> MKSSHHHHHHENLYFQSSSDFVGTHGQLQVIGNQLCNQYGQPIQLRGMSSHGLQWYPQFVNYDSIKWLRDDWGITVFRAAMYTDSQGYISNPSVKNKVIEAVEACIALGIYVIIDWHILADGNPNQYKEQAKDFFREMATRYGNYPNVIYEICNEPNGPVNWNNHIKPYAEEVIPVIRSIDRNNIVIVGTGTWSQDIHDAANNQLSFDNVMYALHFYAGTHGQNLRSRIDYAMSRGAAIFVSEWGVSDASGDGGVFLSQSDVWLDFLNERNVSWVNWSLTHKVESSAALNPGASPNGGWTDANLSPSGRYVKSAMRKNYNPPVPPTTTPTPTPTPTPTPTPTPTPTPTPTPTPTPTPTPTPTPTPTPTPTPTPTPTPTPTPTPTPTPTPTPTPIPEFKTIPGLIQAEDYGNMYGIEVEECSEGGENVGYIDVGDWLDYYVNVQQSGEYTVEFRVASQTDSGRFSLRSGNSSIANFIVPNTGD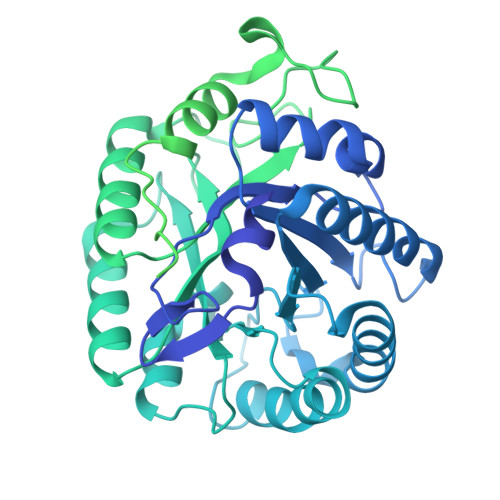WQNWTTISTNVNLYAGEQILRVYADGELFNINWMRFTLNVQPTPTPTPTPTPTPTPTPTPTPTPTPTPTPTPTPTPTPTPTPTPTPTPTPTPTPTPTPEPTPTPEFKTIPGLIQAEDYSDMFGIEVEECSEGGENVGYIDLGDWLDYNVIVEEAGTYTVEFRVASETDLGRFSLRSGESTLASFTVPNTGDWQNWTTISAQVDLDAGEQVLRIYADGELFNINWMKFTLNDITEPSYLLGDVDGDGRINSTDYALVRRFVLEIIDEFPSEYGHLAADVNGDGKIDSLDLILLRRYLLEIIDSF ethyl ({2-[(1,3-benzothiazol-2-ylcarbonyl)amino]thiophen-3-yl}carbonyl)carbamate | 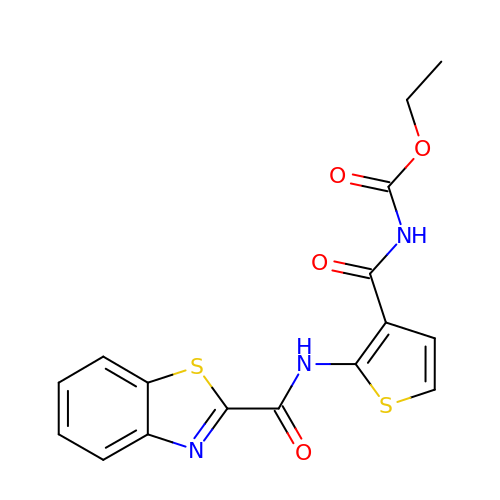C16 H13 N3 O4 S2 | ISNBJLXHBBZKSL-UHFFFAOYSA-N> MKKHHHHHHGPEPTVEDVISQVARAHREIFTYAHDKLGSSPGNFNANHASGSPYPHGRSGRTVQEIWEDFSMSFTPAVREVVEFAKHIPGFRDLSQHDQVTLLKAGTFEVLMVRFASLFNVKDQTVMFLSRTTYSLQELGAMGMGDLLSAMFDFSEKLNSLA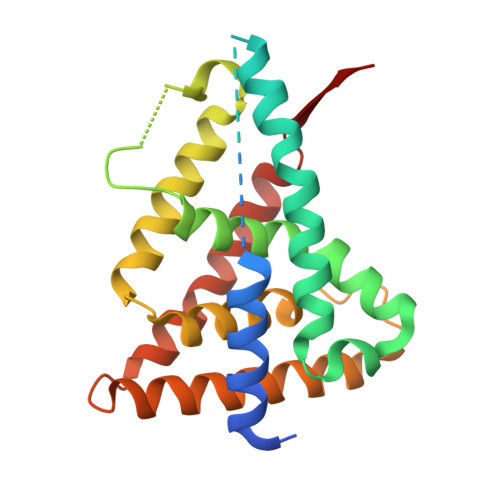LTEEELGLFTAVVLVSADRSGMENSASVEQLQETLLRALRALVLKNRPLETSRFTKLLLKLPDLRTLNNMHSEKLLSFRVDAQ> MEIKRFGRIREVIPLPPLTEIQVESYKKALQADVPPEKRENVGIQAAFKETFPIEEGDKGKGGLVLDFLEYRIGDPPFSQDECREKDLTYQAPLYARLQLIHKDTGLIKEDEVFLGHLPLMTEDGSFIINGADRVIVSQIHRSPGVYFTPDPARPGRYIASIIPLPKRGPWIDLEVEASGVVTMKVNKRKFPLVLLLRVLGYDQETLVRELSAYGDLVQGLLDEAVLAMRPEEAMVRLFTLLRPGDPPKKDKALAYLFGLLADPKRYDLGEAGRYKAEEKLGVGLSGRTLVRFEDGEFKDEVFLPTLRYLFALTAGVPGHEVDDIDHLGNRRIRTVGELMADQFRVGLARLARGVRERMVMGSPDTLTPAKLVNSRPLEAALREFFSRSQLSQFKDETNPLSSLRHKRRISALGPGGLTRERAGFDVRDVHRTHYGRICPVETPEGANIGLITSLAAYARVDALGFIRTPYRRVKNGVVTEEVVYMTASEEDRYTIAQANTPLEGDRIATDRVVARRRGEPVIVAPEEVEFMDVSPKQVFSLNTNLIPFLEHDDANRALMGSNMQTQAVPLIRAQAPVVMTGLEERVVRDSLAALYAEEDGEVVKVDGTRIAVRYEDGRLVEHPLRRYARSNQGTAFDQRPRVRVGQRVKKGDLLADGPASEEGFLALGQNVLVAIMPFDGYNFEDAIVISEELLKRDFYTSIHIERYEIEARDTKLGPERITRDIPHLSEAALRDLDEEGIVRIGAEVKPGDILVGRTSFKGEQEPSPEERLLRSIFGEKARDVKDTSLRVPPGEGGIVVGRLRLRRGDPGVELKPGVREVVRVFVAQKRKLQVGDKLANRHGNKGVV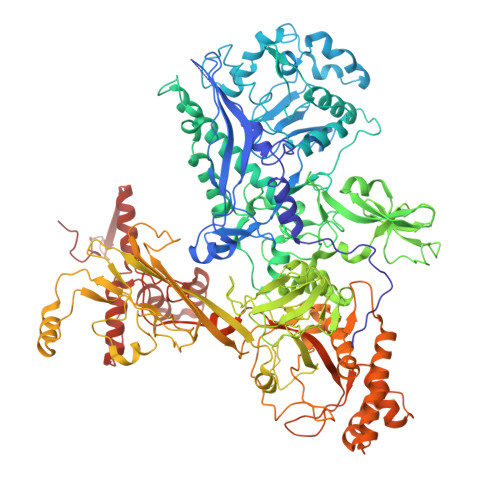AKILPVEDMPHLPDGTPVDVILNPLGVPSRMNLGQILETHLGLAGYFLGQRYISPVFDGATEPEIKELLAEAFNLYFGKRQGEGFGVDKREKEVLARAEKLGLVSPGKSPEEQLKELFDLGKVVLYDGRTGEPFEGPIVVGQMFIMKLYHMVEDKMHARSTGPYSLITQQPLGGKAQFGGQRFGEMEVWALEAYGAAHTLQEMLTIKSDDIEGRNAAYQAIIKGEDVPEPSVPESFRVLVKELQALALDVQTLDEKDNPVDIFEGLASKR>[6x]GSMGLQEEFEEFAEKAKTLPDTISNEDKLLLYGLYKQATVGP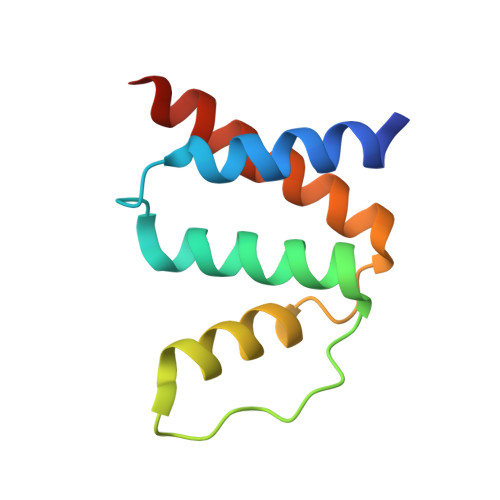VTTGRPGIFNLKDRYKWDAWKAVEGKSKEEAMADYITKVKQLLEEASASTS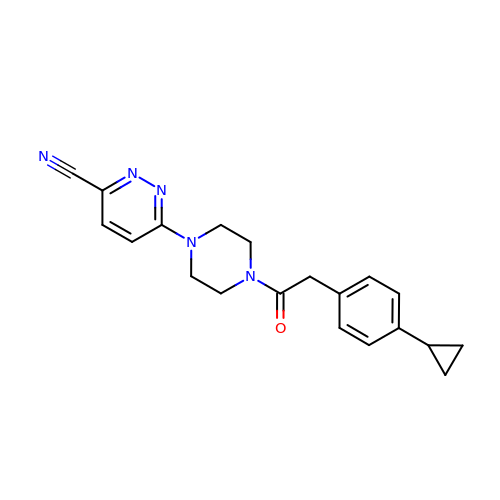6-{4-[(4-cyclopropylphenyl)acetyl]piperazin-1-yl}pyridazine-3-carbonitrile | C20 H21 N5 O | CXSADKGUEBUMLH-UHFFFAOYSA-N4-methyl-~{N}-(4-phenylbutyl)piperidine-1-carboxamide | 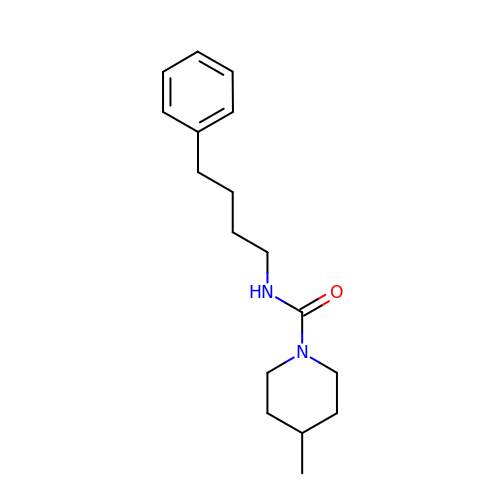C17 H26 N2 O | DHSRHSOXWFKTLE-UHFFFAOYSA-N> LHETSKEPDVSLGSTWLSDFPQAWAETGGMGLAVRQAPLIIPLKATSTPVSIKQYPMSQEARLGIKPHIQRLLDQGILVPCQSPWNTPLLPVKKPGTNDYRPVQDLREVNKRVEDIHPTVPNPYNLLSGLPPSHQWYTVLDLKDAFFCLRLHPTSQPLFAFEWRDPEMGISGQLTWTRLPQGFKNSPTLFDEALHRDLADFRIQHPDLILLQYVDDLLLAATSELDC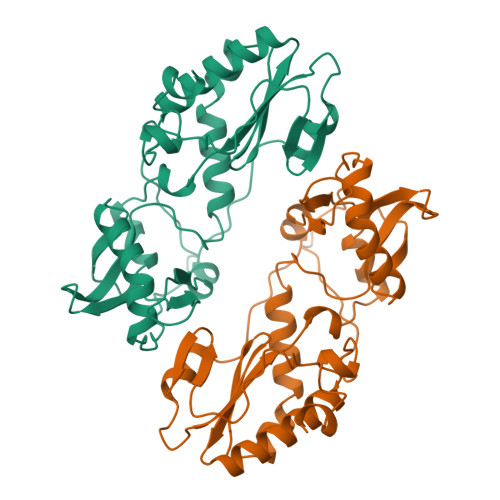QQGTRALLQTLGNLGYRASAKKAQICQKQVKYLGYLLK4-[(5,6-DIMETHYL-2,2'-BIPYRIDIN-3-YL)OXY]-N-(3,4,5-TRIMETHOXYPHENYL)PYRIDIN-2-AMINE | C26 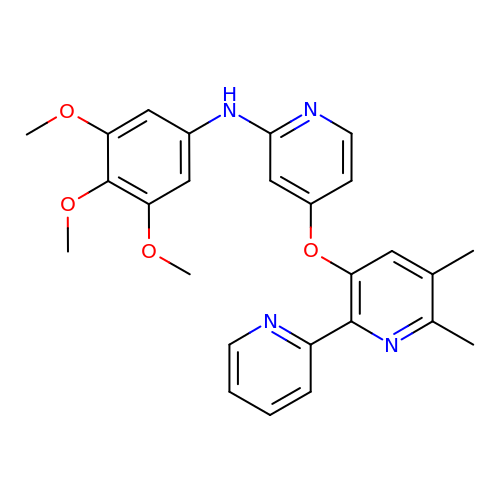H26 N4 O4 | RNLQQRFAMDEKKT-UHFFFAOYSA-N A typical TCS is composed of a sensor histidine kinase (SK) and a cognate response regulator (RR), which are encoded by genes that are often clustered in the genome. Modulated by stimulating signals, an SK first performs an autokinase activity and phosphorylates a conserved histidine in its DHp domain. Here, we sought to determine the crystal structures of a WalK homologue, lpWalK from Lactobacillus plantarum, which shares 60% sequence identity in the DHp and CA domains to our previous solved smVicK structure, in different conformations in the presence of ATP analogues or ADP. The catalytic region of lpWalK contains one DHp domain (amino acids 370–450) and one CA domain (amino acids 450–624).

To obtain ATP-bound states, we crystallized the lpWalK fragment in the presence of the nonhydrolyzable ATP analogues AMPPCP and AMPPNP. In addition, the γP of ATP was visible when lpWalK was co-crystallized with AMPPCP but not AMPPNP. Interestingly, the interaction between Lys476 and Ala406 in lpWalK is not found in smVicK as Lys476 is substituted by Gln301. Together, our data indicate that WalK adopts a closed structure in the presence of ATP analogues or ADP, which is characterized by the asymmetric positioning of the two CA domains; only one monomer of the dimer switches to a closed conformation while the other one remains open. Only one monomer folds into a closed state through an ∼58° rotation, while the other monomer remains open. ATP/ADP fits into the active site of the CA domain through extensive interactions involving the N box and the G1 and G2 loops. We have found that ATP/ADP interacts with His391 in the DHp domain through hydrogen bonds in the closed lpWalK. A magnesium ion was not identified in the ATP/ADP-binding pocket of the closed lpWalK structures. Two coordinations by the hydroxyl groups of βP and γP are lost in our lpWalK structure bound to AMPPCP, which makes lpWalK unable to chelate Mg2+ stably. The DHp domain is sandwiched between two CA domains. In the open WalK structure the DHp is completely symmetric, with two straight α1 helices, whereas in the closed WalK state it is asymmetric, as characterized by helical bending in one α1 but not the other.

>HDVTEQQKIDNDRKQFVSNVSHELRTPLTSLRSYIEALSDGAWKDPEVAPGFLKVTQEETDRMIRMINELLSLSRMDSGTTRVDMELVNINEMFNYVLDRFDMILKKDDNPAKYYTIKREFTKRDLWVEIDTDKFTQVLDNIMNNAIKYSPDGGVVTCRLLETHNQVIISISDQGLGIPRADLGHVFDRFFRVDKARSRAQGGTGLGLAISKEVVQMLGGRIWVDSVEGKGSTFYISLPYEPYEEEDLWDDDSQA[2x]> MAEPWGNELASAAARGDLEQLTSLLQNNVNVNAQNGFGRTALQVMKLGNPEIARRLLLRGANPDLKDRTGFAVIHDAARAGFLDTLQTLLEFQADVN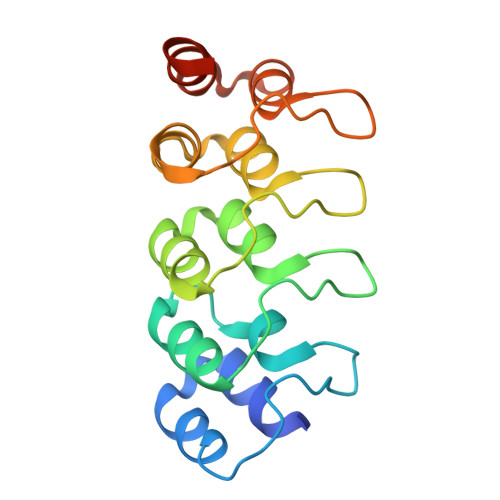IEDNEGNLPLHLAAKEGHLRVVEFLVKHTASNVGHRNHKGDTACDLARLYGRNEVVSLMQANGAGGATNLQ>[4x]MTDLNTPESTSKPVWEHFDHVEPGIRRRIAVADPEIKEYLDGMLARIASHRGVEHPFLNAYRTTALDPEQERHLFSECYYFFRY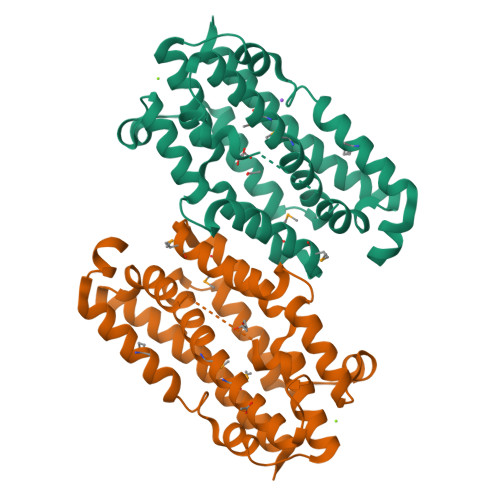LPFYITGMAVKTRDEMILREIILNVADEVGSDPTHSTLFADFLARIGIDKEHLDGYQPLEVTRQLNDGIRHLYTETSINKALGALYADETMSSIMVSKINDGLRNQGYDDDLRHFWQLHIDVEVGHSNSVFNAIAPYVGSKAARAEFEEGVFEFLGLVERYWDGVRELVGIGK>[2x]ATCYCRT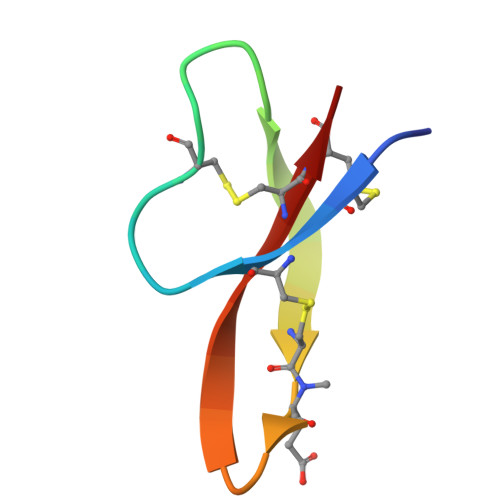GRCATRESLSGVCXISGRLYRLCCR> MGNQDKSKETSELDDLALPRSIIMRLVKGVLPEKSLVQKEALKAMINSATLFVSFLTSASGEIATNNNRKILMPQDVLNALDEIEYPEFSKTLKKHLEAYELALKEK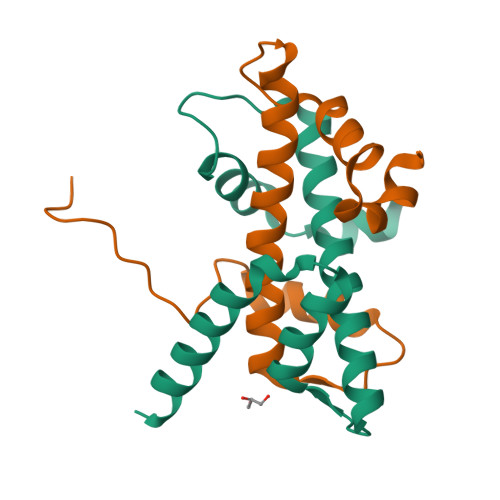RLKLPNVSDVDNRKKAKIDAHDTTPLDEEKDELEEERIAEDIAQNEVEQNIDDVEDLEEVNDTLDANAESPQIETIHLTDATGNPIEDSSESDSEESLQLNDSSAAAENLYFQGLEDYKDDDDKHHHHHHHHHH;> GPLGSMEKTYGKTVLPLSRVKRIIKQDEDVHYCSNASALLISVATELFVEKLATEAYQLAKLQKRKGIRYRDVEDVVRKDDQFEFLSDLFSI> AEG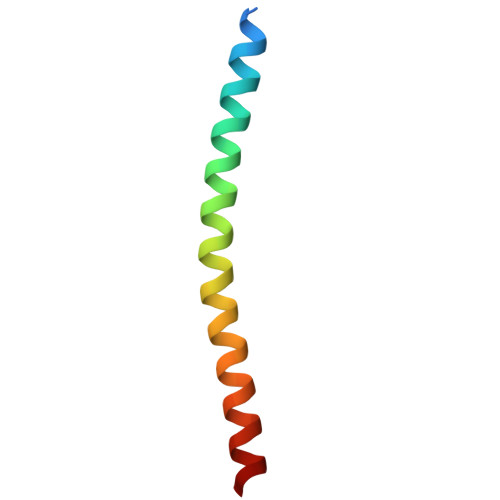DDPAKAAFDSLQASATEMIGYAWAMVVVIVGATIGIKLFKKFTSKAS> GSHMNGLIYAVGGYDGTGYNTHLNSVEAYDPERNEWSLVAPLSTRRSGVGVAVLNGLIYAVGGYDGTGYNTHLNSVEAYDPERNEW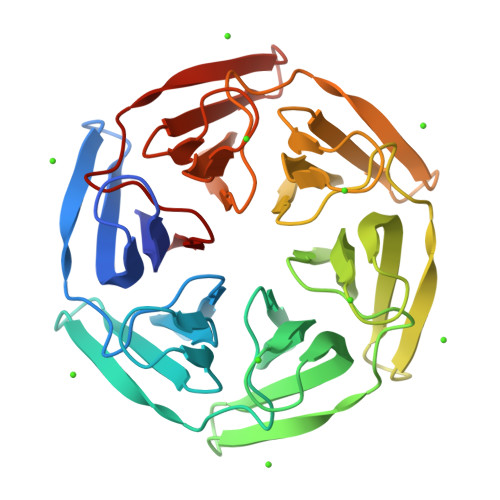SLVAPLSTRRSGVGVAVLNGLIYAVGGYDGTGYNTHLNSVEAYDPERNEWSLVAPLSTRRSGVGVAVLNGLIYAVGGYDGTGYNTHLNSVEAYDPERNEWSLVAPLSTRRSGVGVAVLNGLIYAVGGYDGTGYNTHLNSVEAYDPERNEWSLVAPLSTRRSGVGVAVLNGLIYAVGGYDGTGYNTHLNSVEAYDPERNEWSLVAPLSTRRSGVGVAVL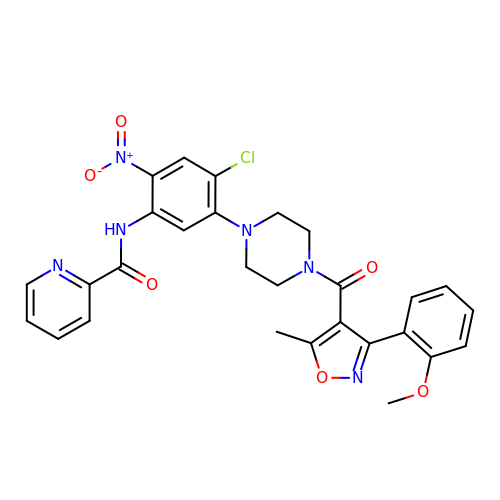N-[4-chloranyl-5-[4-[[3-(2-methoxyphenyl)-5-methyl-1,2-oxazol-4-yl]carbonyl]piperazin-1-yl]-2-nitro-phenyl]pyridine-2-carboxamide | C28 H25 Cl N6 O6 | QSXDDWUUADOGGK-UHFFFAOYSA-N In these yeast cells, around 50 AFs and several snoRNAs, such as U3, U14 and snR30, associate co-transcriptionally with the 35S pre-RNA to form the first pre-ribosomal particle known as 90S or the SSU-processome. The UTP-B complex consists of Utp6p, Utp12p/Dip2p, Utp13p, Utp18p, Utp21p, and Pwp2p/Utp1p5. Pwp2p is a protein subunit of UTP-B and essential for the stable assembly of a large set of proteins forming the SSU-processome. We report the structure of the N-terminal domain of Pwp2p, which exhibits a prototypical tandem WD40 repeat (tWD).

The WD-repeat-containing region of Pwp2p (residues 1–716) was subcloned, produced and purified as described in the Methods section. The purified protein was crystallized, and X-ray diffraction data were collected up to 2.54 Å resolution. Over the 716 residues of the construct, the final model comprises 608 residues (from residue 4 to 707). Pwp2p (1–716) contains two canonical WD40 domains, WD1 and WD2. Each WD domain is a seven-bladed β-propeller composed of four anti-parallel β-strands. The first WD-repeat domain (WD1) is composed of residues 12–343. The second WD-repeat domain (WD2) is composed of residues 4–11 and 344–706. The connection between the two WD domains is ensured by residues 12–14 and 342–346 in addition to the external β-strands of blade 1 of each WD domain, and the loop connecting blade 1 and blade 2. The two WD domains form an angle of approximately 30°. Several patches of conserved residues were identified, some of which were spanning an extended area over WD1 and WD2.

> MGSSHHHHHHSSGTGSGENLYFQGHMKSDFKFSNLLGTVYRQGNITFSDDGKQLLSPVGNRVSVFDLINNKSFTFEYEHRKNIAAIDLNKQGTLLISIDEDGRAILVNFKARNVLHHFNFKEKCSAVKFSPDGRLFALASGRFLQIWKTPDVNKDRQFAPFVRHRVHAGHFQDITSLTWSQDSRFILTTSKDLSAKIWSVDSEEKNLAATTFNGHRDYVMGAFFSHDQEKIYTVSKDGAVFVWEFTKRPSDDDDNESEDDDKQEEVDISKYSWRITKKHFFYANQAKVKCVTFHPATRLLAVGFTSGEFRLYDLPDFTLIQQLSMGQNPVNTVSVNQTGEWLAFGSSKLGQLLVYEWQSESYILKQQGHFDSTNSLAYSPDGSRVVTASEDGKIKVWDITSGFCLATFEEHTSSVTAVQFAKRGQVMFSSSLDGTVRAWDLIRYRNFRTFTGTERIQFNCLAVDPSGEVVCAGSLDNFDIHVWSVQTGQLLDALSGHEGPVSCLSFSQENSVLASASWDKTIRIWSIFGRSQQVEPIEVYSDVLALSMRPDGKEVAVSTLKGQISIFNIEDAKQVGNIDCRKDIISGRFNQDRFTAKNSERSKFFTTIHYSFDGMAIVAGGNNNSICLYDVPNEVLLKRFIVSRNMALNGTLEFLNSKKMTEAGSLDLIDDAGENSDLEDRIDNSLPGSQRGGDLSTRKMRPEVRVTSVQFSPTANAFAAASTEGLLIYSTNDTILFDPFDL>SQIGLFSKICRVTIKTLHYYNKIGLLVPAYINPDNGYRFYTSDQLMKFHQIASLRQLGFTITEIVTLTQDENSCHIIERRRLEIQKQIRDMADMLSRINHYLQHKKKERIMLYQAALKEIPECIVYSKRFIVPDFSSYIKLIPPIGQEVMKANPGLTLTTPAYCFTLYHDKEYKEKNMDVEFCEAVNDFGKNEGNIIFQVIPAITAVTVIHKGPYDSLRNAYIYLMQWVEDNGYLLTNSPRESYIDGIWNKQDSAEWMTEIQFPVEKV[2x]

Bacterial RNA polymerase (RNAP) holoenzyme initiates transcription by recognizing the conserved –35 and –10 promoter elements that are optimally separated by a 17-bp spacer. The MerR family of transcriptional regulators activate suboptimal 19–20 bp spacer promoters in response to myriad cellular signals, ranging from heavy metals to drug-like compounds. Here we report one crystal structure of a multidrug-sensing MerR family regulator EcmrR and nine cryo-electron microscopy structures that capture the EcmrR-dependent transcription process from promoter opening to initial transcription to RNA elongation. These structures reveal that EcmrR is a dual ligand-binding factor that reshapes the suboptimal 19-bp spacer DNA to enable optimal promoter recognition, sustains promoter remodeling to stabilize initial transcribing complexes, and finally dissociates from the promoter to reverse DNA remodeling and facilitate the transition to elongation.

An EcmrR dimer binds to promoter DNA between the –35 and –10 elements and introduces a 58° kink in the DNA backbone, facilitated by A:T base unpairing at the center of the pseudo-palindromic sequence recognized by the EcmrR dimer. In addition, EcmrR under-twists the 19-bp spacer DNA by 82° relative to an ideal B-form 19-bp DNA and realigns the –35 and –10 elements for recognition by σ4 and σ2 domains, respectively. The spacer DNA conformation in EcmrR-RPo is highly similar to those observed in the structures of BmrR-TAC and CueR-TAC, reflecting a shared DNA remodeling mechanism by MerR family regulators. EcmrR-promoter binding is mediated by both base-specific hydrogen bonds and backbone interactions. The characteristic HTH motif and a following β-hairpin straddle the DNA backbone. K16 from α2 and Y38 from the β1–β2 loop insert into the major and minor grooves, respectively, and make base-specific hydrogen bonds. Backbone phosphate interactions are mainly contributed by H19, Y21, R39, R56 and several mainchain nitrogen atoms. Intriguingly, we observed strong extra density in another hydrophobic pocket (hereinafter designated site II) in the cryo-EM maps of EcmrR-RPo and EcmrR-RPitc-4nt. The density likely corresponds to the tetracyclic sterol head of CHAPSO, which is routinely used in cryo-EM sample preparation of bacterial RNAP complexes to alleviate preferred orientation problems.>MRSTKVIHI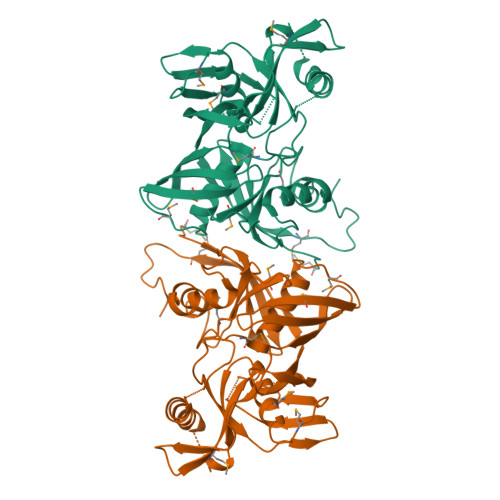VGCHAEGEVGDVIVGGVAPPPGETVWEQSRFIANDETLRNFVLNKPRGGVFRHVNLLVPPKDPRAQMGFIIMEPADTPPMSGSNSICVSTVLLDSGIIAMQEPVTHMVLEAPGGIIEVEAECRNGKAERISVRNVPSFADRLDAPLDVTGLGTIMVDTAYGGDSFVIVDAAQIGMKIEPGQARELAEIGVKITKAANEQLGFRHPERDWRHISFCQITEPVTREGDVLTGVNTVAIRPAKFDRSPTGTGCSARMAVLHAKGQMKAGERFIGKSVLGTEFHCRLDKVLELGGKPAISPIISGRAWVTGTSQLMLDPSDPFPHGYRLSDTWPRDELEHHHHHH[2x]>GSHMKPASFMTSICDERGQELIYAGMPITEVF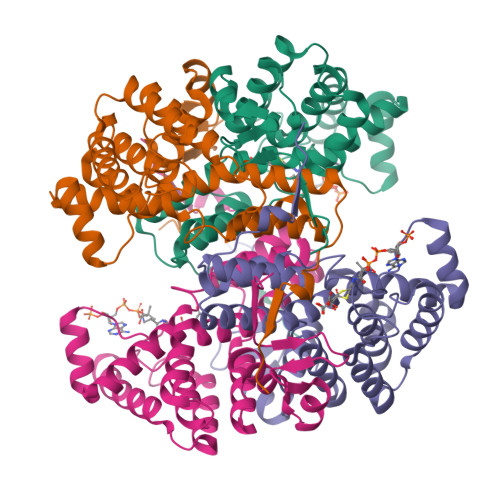KEEMGIGGVLGLLWFQKRLPKYSCQFIEMCLMVTADHGPAVSGAHNTIICARAGKDLVSSLTSGLLTIGDRFGGALDAAAKMFSKAFDSGIIPMEFVNKMKKEGKLIMGIGHRVKSINNPDMRVQILKDYVRQHFPATPLLDYALEVEKITTSKKPNLILNVDGLIGVAFVDMLRNCGSFTREEADEYIDIGALNGIFVLGRSMGFIGHYLDQKRLKQGLYRHPWDDISYVLPEHMSM[4x]> MNQQKSLTLIVALTTSYGIGRSNSLPWKLKKEISYFSRVTSFVPTFDSFESMNVVLMGRKTWESIPLQNRPLKGRINVVITRNESLDLGNGIHSAKSLDHALELLYRTYGSESSVQINRIFVIGGAQLYKAAMD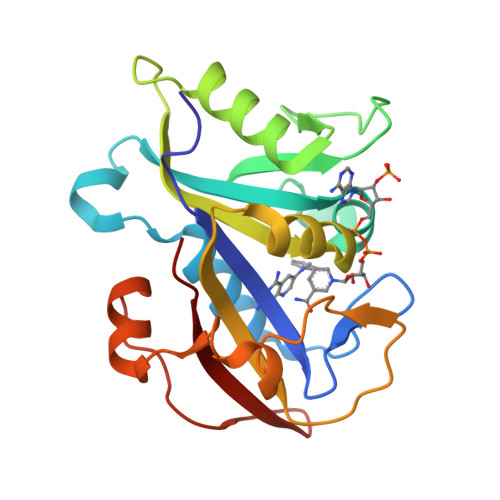HPKLDRIMATIIYKDIHCDVFFPLKFRDKEWSSVWKKEKHSDLESWVGTKVPHGKINEDGFDYEFEMWTRDL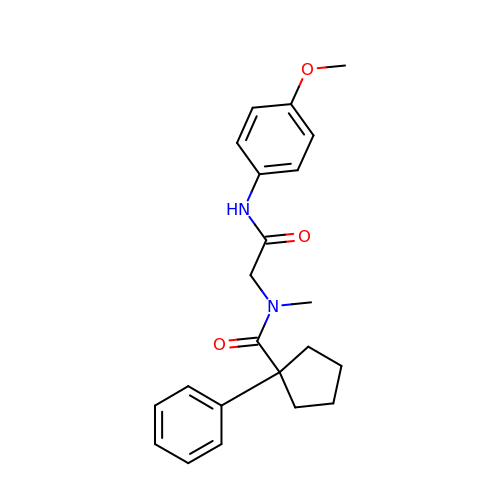N-[2-(4-methoxyanilino)-2-oxoethyl]-N-methyl-1-phenylcyclopentane-1-carboxamide | C22 H26 N2 O3 | DKCHMKRLQSFONS-UHFFFAOYSA-N>MGGSHHHHHHGLVPRGSKILISGGAGYIGSHTLRQ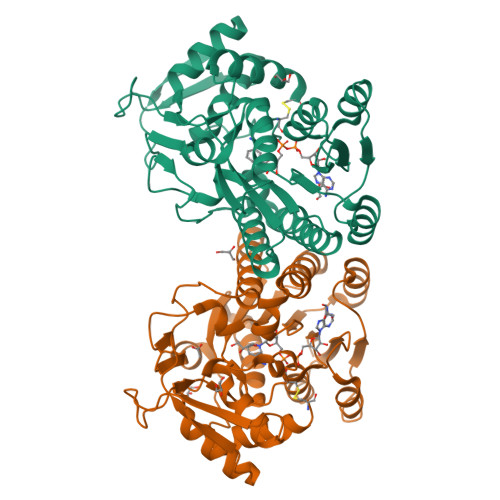FLKTDHEICVLDNLSKGSKIAIEDLAATRAFKFFEQDLSDFQGVKALFEREKFDAIVHFAASIEVFESMQNPLKYYMNNTVNTTNLIETCLQTGVNKFIFSSTAATYGEPQTPVVSETSPLAPINPYGRSKLMSEEVLRDASMANPEFKHCILRYFNVAGACMDYTLGQRYPKATLLIKVAAECAAGKRDKLFIFGDDYDTKDGTCIRDFIHVDDISSAHLAALDYLKENESNVFNVGYGHGFSVKEVIEAMKKVSGVDFKVELAPRRAGDPSVLISDASKIRNLTSWQPKYDDLELICKSAFDWEKQC[2x]>[4x]VVCREASHAGSWYTASGPQLNAQLEGWLSQVQSTKRPARAIIAPHAGYTYCGSCAAHAYKQVDPSITRRIFILGPSHHVPLSRCALSSVDIYRTPLYDLRIDQKIYGELWKTGMFERMSLQTDEDEHSIEMHLPYTAKAMESHKDEFTIIPVLVGALSESKEQEFGKLFSKYLADPSNLFVVSSDFCHWGQ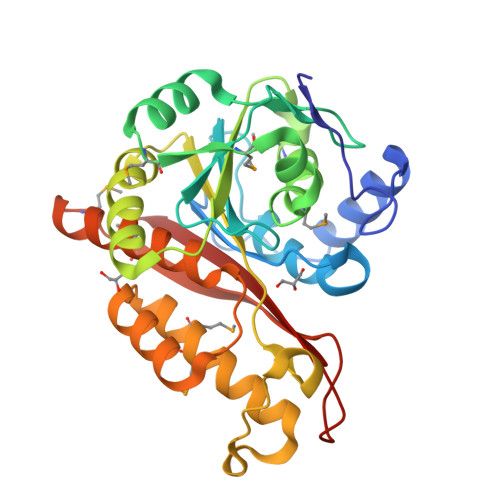RFRYSYYDESQGEIYRSIEHLDKMGMSIIEQLDPVSFSNYLKKYHNTICGRHPIGVLLNAITELQKNGMNMSFSFLNYAQSSQCRNWQDSSVSYAAGALTVH3-(4-hydroxypiperidin-1-yl)benzene-1,2-dicarboxylic 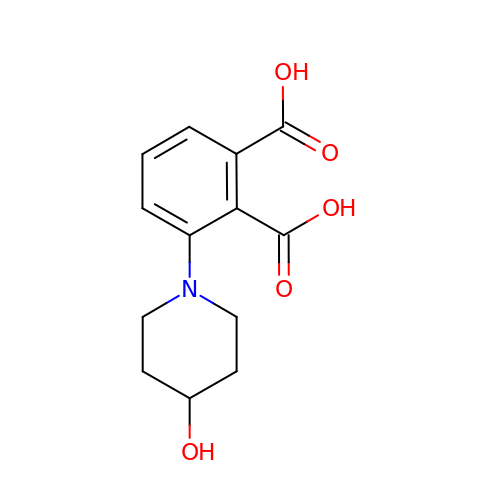acid | C13 H15 N O5 | WHCKCCDPUOWOSW-UHFFFAOYSA-N>[4x]MSLRSIFWDDGLKLIDQTKLPEKLEVIECRNVEELADAIKKLAVRGAPALEAAGAYGIALAAREREFADVDELKEHLKKAADFLASTRPTAVNLFVGIERALNAALKGESVEEVKELALREAEKLAEEDVERNRKMGEYGAELLEDGDVVLTYCNAGRLATVDWGTALGVVRSAVEQGKEIRVIACETRPL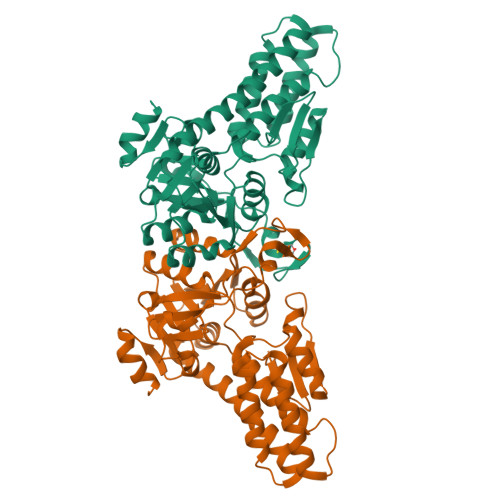NQGSRLTCWELMEDGIDVTLITDSMVGIVMQKGMVDKVIVGADRIVRDAVFNKIGTYTVSVVAKHHNIPFYVAAPKATFDWERTAKDVVIEERPREELIFCGKRQIAPLNVKVYNPAFDPTPLENVTALITEYGVIYPPYEVNVPKVLKFEGGSHHHHHH> MSAVALPRVSGGHDEHGHLEEFRTDPIGLMQRVRDELGDVGTFQLAGKQVVLLSGSHANEFFFRAGDDDLDQAKAYPFMTPIFGEAVVFDASPERRKEMLHNAALRGEQMKGHAATIEDQVRRMIADWGEAGEIDLL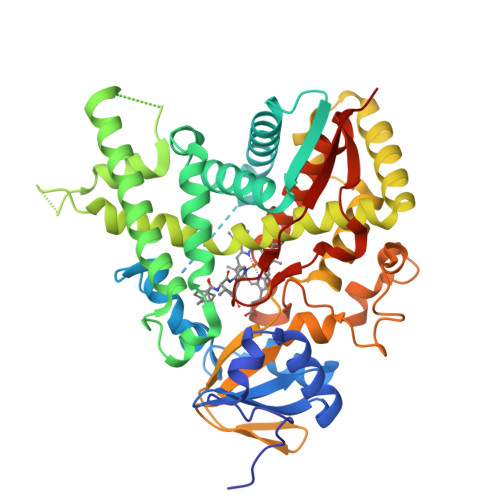DFFAELTIYTSSACLIGKKFRDQLDGRFAKLYHELERGTDPLAYVDPYLPIESFRRRDEARNGLVALVADIMNGRIANPPTDKSDRDMLDVLIAVKAETGTPRFSADEITGMFISMMFAGHHTSSGTASWTLIELMRHRDAYAAVIDELDELYGDGRSVSFHALRQIPQLENVLKETLRLHPPLIILMRVAKGEFEVQGHRIHEGDLVAASPAISNRIPEDFPDPHDFVPARYEQPRQEDLLNRWTWIPFGAGRHRCVGAAFAIMQIKAIFSVLLREYEFEMAQPPESYRNDHSKMVVQLAQPAAVRYRRRTGVHHHH>[2x]GPGSGQLLFANFNQ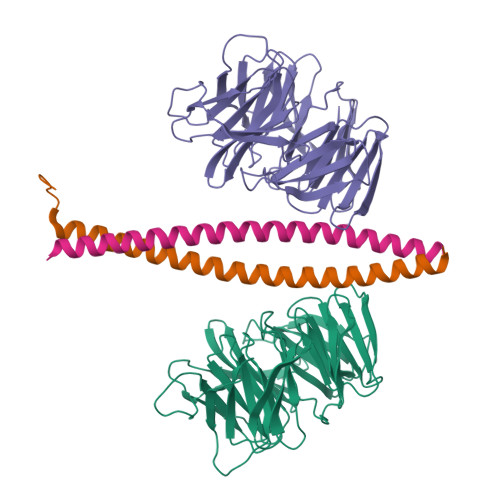DNTSLAVGSKSGYKFFSLSSVDKLEQIYECTDTEDVCIVERLFSSSLVAIVSLKAPRKLKVCHFKKGTEICNYSYSNTILAVKLNRQRLIVCLEESLYIHNIRDMKVLHTIRETPPNPAGLCALSINNDNCYLAYPGSATIGEVQVFDTINLRAANMIPAHDSPLAALAFDASGTKLATASEKGTVIRVFSIPEGQKLFEFRRGVKRCVSICSLAFSMDGMFLSASSNTETVHIFKLETVKEQGRAFATVRLPFCGHKNICSLATIQKIPRLLVGAADGYLYMYNLDPQEGGECALMKQHRLDGSLE;>GPGSMQMNEAKIAECLQTISDLETECLDLRTKLCDLERANQTLKDEYDALQITFTALEGKLRKTTEENQ[2x]>[4x]MGSSHHHHHHSSGRENLYFQGHMKTFEVMIQTDSKGYLDAKFGGNAPKAFLNSNGLPTYSPKISWQKVEGAQSYALELIDHDAQKVCGMPFVHWVVGNIAHNVLE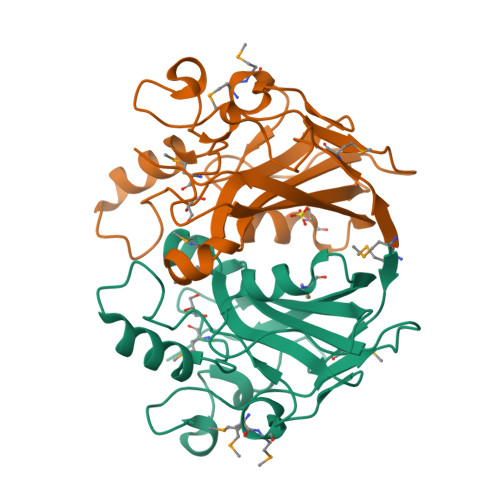ENASMMDKRIVQGVNSLTQGFIRSPLNESEKQRSNLNNSVYIGPMPPNGDHHYLIQVYALDIPKLALKAPFFLGDLHDKMRNHIIAIGRKEFLYKQFVRKGS> KHHVFPSFHGADVRKTILSHILESFRRKGIDPFIDNNIERSKSIGHELKEAIKGSKIAIVLLSKNYASSSWCLDELAEIMKCRELLGQIVMTIFYEVDPTDIKKQTGEFGKAFTKTCKGKTKEYVERWRKALEDVATIAGYHSH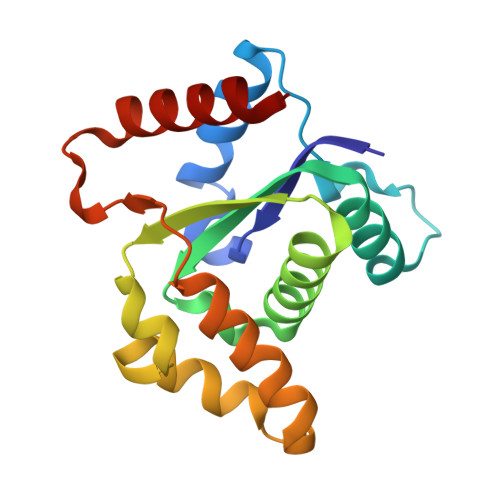KWRNEADMIEKIATDVSNMLN> MAPSMIPFTIKLKTCLKMCIQRLRYAQEKQQAIAKQSRRQVAQLLLTNKEQKAHYRVETLIHDDIHIELLEILELYCELLLARVQVINDISTEEQLVKEHMDDGINEAIRSLIYAILFVDEVKELSQLKDLMA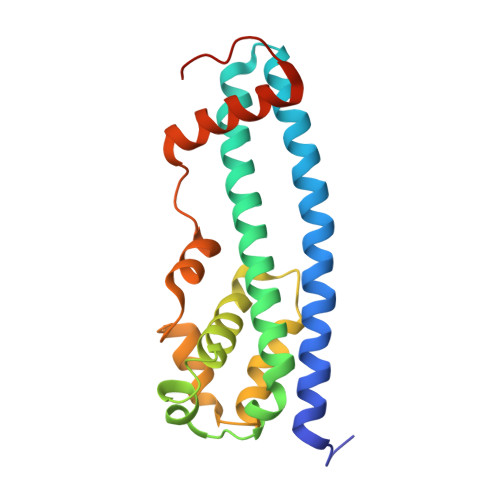WKINVEFVNGVIADHIDVPEKIIKKCSPSVPKEELVDLYLKEIAKTYDVPYSKLENSLSS> STRDYEIQRERIELGRCIGEGQFGDVHQGIYMSPENPAMAVAIKTCKNCTSDSVREKFLQEALTMRQFDHP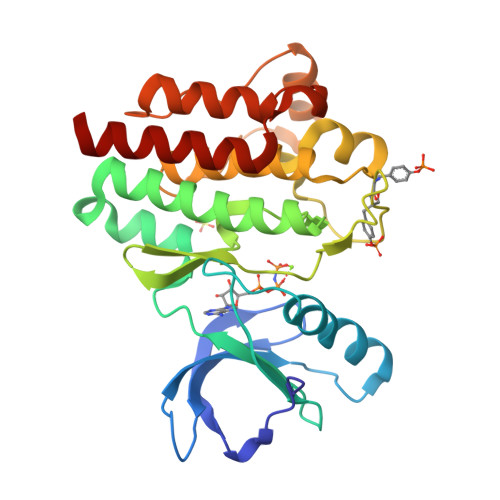HIVKLIGVITENPVWIIMELCTLGELRSFLQVRKFSLDLASLILYAYQLSTALAYLESKRFVHRDIAARNVLVSSNDCVKLGDFGLSRYMEDSTYYKASKGKLPIKWMAPESINFRRFTSASDVWMFGVCMWEILMHGVKPFQGVKNNDVIGRIENGERLPMPPNCPPTLYSLMTKCWAYDPSRRPRFTELKAQLSTILEEEKLQ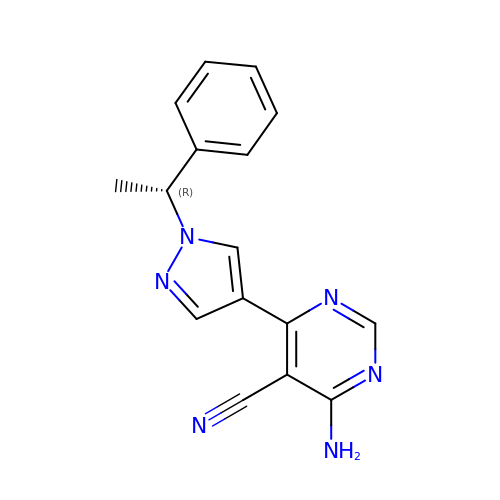4-azanyl-6-[1-[(1~{R})-1-phenylethyl]pyrazol-4-yl]pyrimidine-5-carbonitrile | C16 H14 N6 | YHDDGKWKOCFLDB-LLVKDONJSA-N1-chloranyl-4-methyl-benzene | C7 H7 Cl | 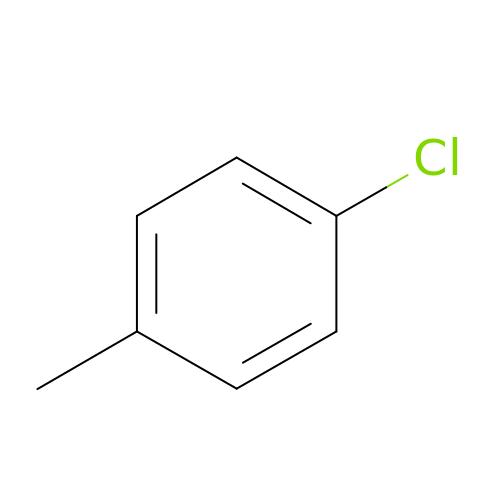NPDACUSDTOMAMK-UHFFFAOYSA-N Here we report the use of single particle cryo-EM to identify multiple proteins from three enriched heterogeneous fractions prepared from human liver mitochondrial lysate. Using this approach, we were able to simultaneously identify and solve cryo-EM structures of nine different human mitochondrial enzymes: short chain acyl-CoA dehydrogenase (SCAD), medium chain acyl-CoA dehydrogenase (MCAD), isovaleryl-CoA dehydrogenase (IVD), delta (3, 5)-delta dienoyl-CoA isomerase (ECH1), aspartate aminotransferase (GOT2), glutamate dehydrogenase (GLUD1), mitochondrial superoxide dismutase 2 (SOD2), catalase (CAT), and mitochondrial aldehyde dehydrogenase (ALDH2). Functionally, the three acyl-CoA dehydrogenases—SCAD, MCAD and IVD—are involved in beta oxidation and amino acid catabolism. Finally, SOD2, CAT, and ALDH2 are all involved in clearing toxic byproducts of oxidative respiration.

SOD2 is a manganese-binding member of the SOD family that is expressed in the mitochondria and catalyzes the oxidation of two O2− ions to molecular O2 and H2O2 (46). Our BaR methodology classified a total of 50,014 single particle projections for the SOD2 class. Based on these projections, we constructed a high-resolution density map of 2.91 Å. The global architecture of SOD2 is a homotetramer formed by a dimer of dimers. Similarly to existing crystal structures, each subunit of SOD2 contains an N-terminal domain primarily consisting of two long α helices and a C-terminal domain made up of a core three stranded β sheet flanked by a set of six α helices. A central cavity is formed by the interface of each subunit’s β-sheet core, while dimer interfaces consist of α-helical bundles from the N-terminal domains. Elements of both domains contribute to the Mn2+-binding site for each subunit. Specifically, this cavity is formed by the H50 and H98 from the N-terminal domain and D183 and H187 from the C-terminal domain.

>[4x]MLSRAVCGTSRQLAPVLGYLGSRQKHSLPDLPYDYGALEPHINAQIMQLHHSKHHAAYVNNLNVTEEKYQEALAKGDVTAQIALQPALKFNGGGHINHSIFWTNLSPNGGGEPKGELLEAIKRDFGSFDKFKEKLTAASVGVQGSGWGWLGFNKERGHLQIAACPNQDPLQGTTGLIPLLGIDVWEHAYYLQYKNVRPDYLKAIWNVINWENVTERYMACKK> GSHMLTKQQIRYCLDEMAKMFPDAHCELVHRNPFELLIAVVLSAQCTDALVNKVTKRLFEKYRTP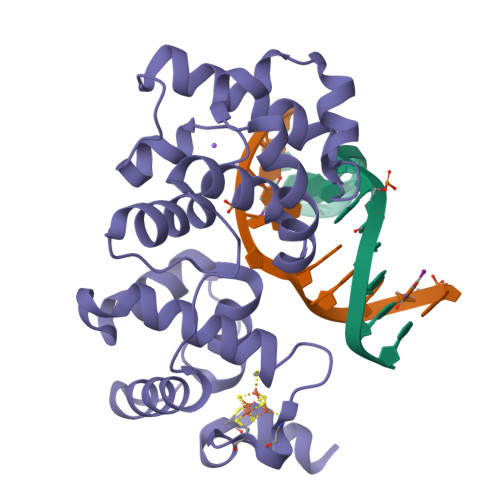HDYIAVPLEELEQDIRSIGLYRNKARNIQKLCAMLIDKYNGEVPRDRDELMKLPGVGRKTANVVVSTAFGVPAIAVDTHVERVSKRLGFCRWDDSVLEVEKTLMKIIPKEEWSITHHRMIFFGRYHCKAQSPQCPSCPLLHLCREGKKRMRKREEKAANQK> ASHMQRIAVTAEGPGLDGLVDPRFGRAAGFVVVDAATMAAEYVDNG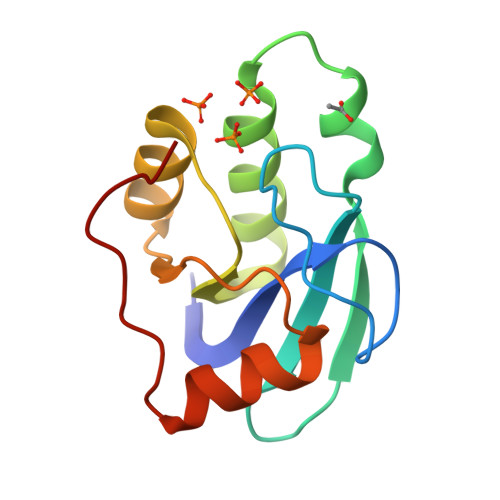ASQTLSHGAGINAAQVLAKSGAGVLLTGYVGPKAFQALQAAGIKVGQDLEGLTVRQAVQRFLDGQVPMAAGPNK>[8x]AADVYVPDEWEVAREKITMSRELGQGSFGMVYEGVAKGVVKDEPETRVAIKTVNEAASMRERIEFLNEASVMKEFNCHHVVRLLGVVSQGQPTLVIMELMTRGDLKSYLRSLRPAMANNPVLAPPSLSKM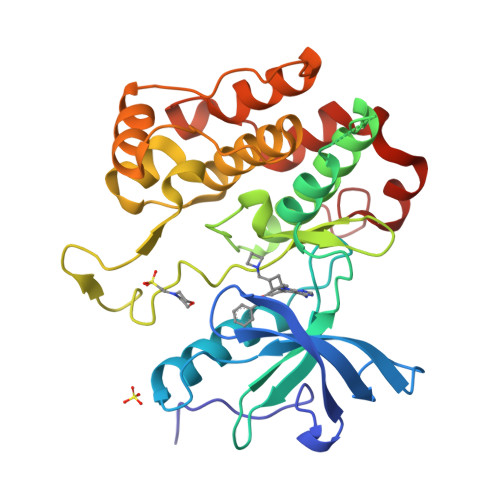IQMAGEIADGMAYLNANKFVHRDLAARNCMVAEDFTVKIGDFGMTRDIYETDYYRKGGKGLLPVRWMSPESLKDGVFTTYSDVWSFGVVLWEIATLAEQPYQGLSNEQVLRFVMEGGLLDKPDNCPDMLFELMRMCWQYNPKMRPSFLEIISSIKEEMEPGFREVSFYYSEENK> GACEQNEDWVVNEPMQSFEENPEYAPLNTIPDWVSEKVTPKEYELWRTMSSRYEINYSFLKKDISEKRKKEIYDCINNICERIEKGQINKYEGFLNIADEDGTTLSDSQYFGRIATRSPEGGAEYKTNGCTLYTHSLGPYIKAAVTYKKSDDDV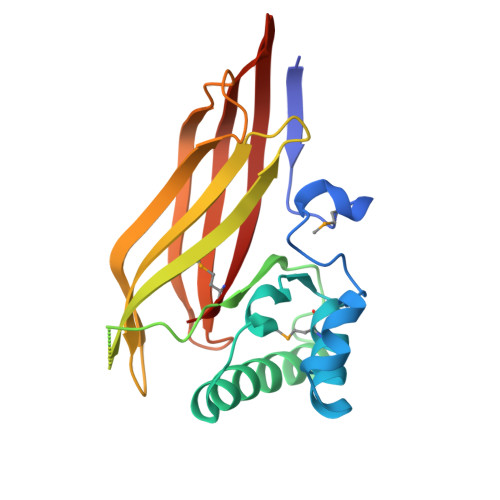TITSSSVYTGSPYLGNDPSFSGASSVSYDKDKKLIAASCSGTLSFKDGSRKVEVTVQKTGFMIP3-DEOXY-D-LYXO-HEXONIC ACID | C6 H12 O6 | 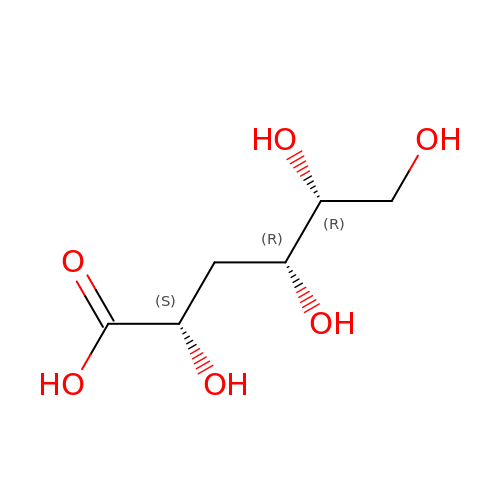YGMNHEPVTNXLLS-MROZADKFSA-N> TASADQIQECFQIFDKDNDGKVSIEELGSALRSLGKN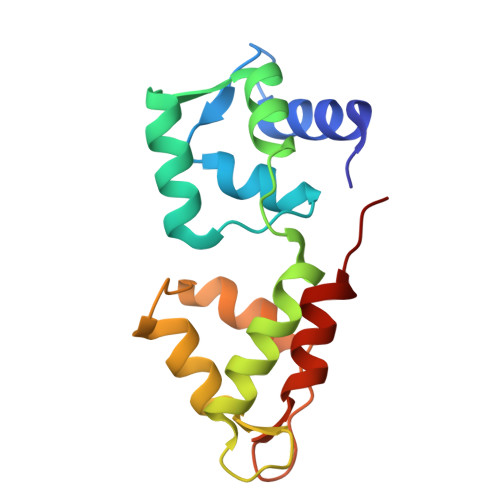PTNAELNTIKGQLNAKEFDLATFKTVYRKPIKTPTEQSKEMLDAFRALDKEGNGTIQEAELRQLLLNLGDALTSSEVEELMKEVSVSGDGAINYESFVDMLVTGYPLA METHYL 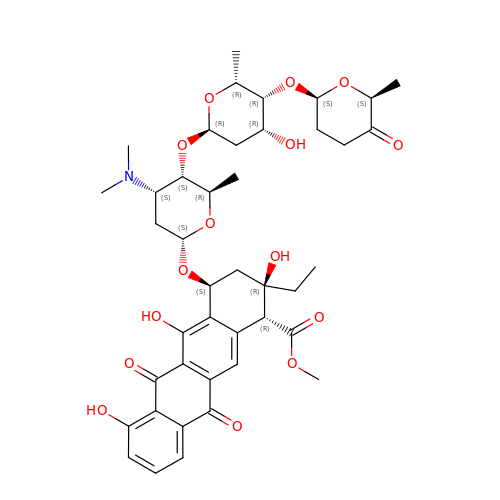(2S,4R)-2-ETHYL-2,5,7-TRIHYDROXY-6,11-DIOXO-4-{[2,3,6-TRIDEOXY-4-O-{2,6-DIDEOXY-4-O-[(2S,6S)-6-METHYL-5-OXOTETRAHYDRO-2H-PYRAN-2-YL]-ALPHA-D-LYXO-HEXOPYRANOSYL}-3-(DIMETHYLAMINO)-D-RIBO-HEXOPYRANOSYL]OXY}-1,2,3,4,6,11-HEXAHYDROTETRACENE-1-CARBOXYLATE | C42 H53 N O15 | USZYSDMBJDPRIF-JAFKFOJZSA-N> GGUUAAGUUAGGUUUGUGGUUGAAAGUCGAUGCCAGUCGCAGGCAAAACGAUCCACGUAAGUUAAACAAAGUUUUAAUGAGCAUGGUGCGGCUUAGAAGUAAG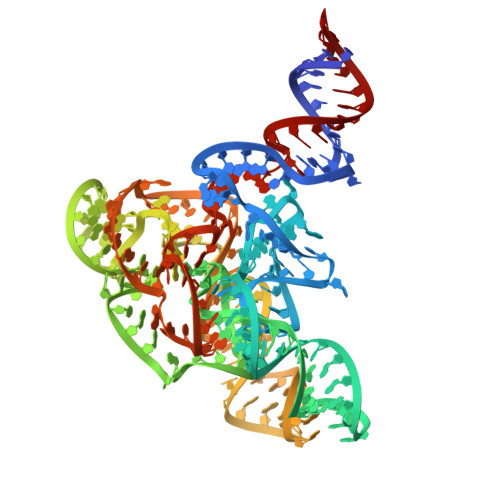UCCUGCCGCUUUAGGCGAGAGUAUUAGUAGUGAGAGGGUAAUUCCGGGUAGCGAAACUUCCAGCAGGCGAGUGUGGGGUCAAAGACCAGGUCAACUAACUUA>[4x]MKAVQYTEIGSEPVVVDIPTPTPGPGEILLKVTAAGLCHSDIHVMDMPAAQYAYGLPLTLGHEGVGTVAELGEGVTGFGVGDAVAVYGPWGCGACHA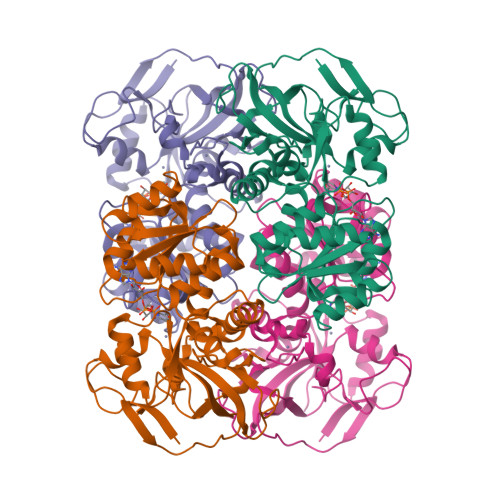CARGRENYCTRAADLGITPPGLGSPGSMAEYMIVDSARHLVPIGDLDPVAAAPLTDAGLTPYHAISRVLPLLGPGSTAVVIGVGGLGHVGIQILRAVSAARVIAVDLDDDRLALAREVGADAAVKSGAGAADAIRELTGGQGATAVFDFVGAQSTIDTAQQVVAVDGHISVVGIHAGAHAKVGFFMIPFGASVVTPYWGTRSELMEVVALARAGRLDIHTETFTLDEGPAAYRRLREGSIRGRGVVVPTSHHHHH> LQFAYKDPE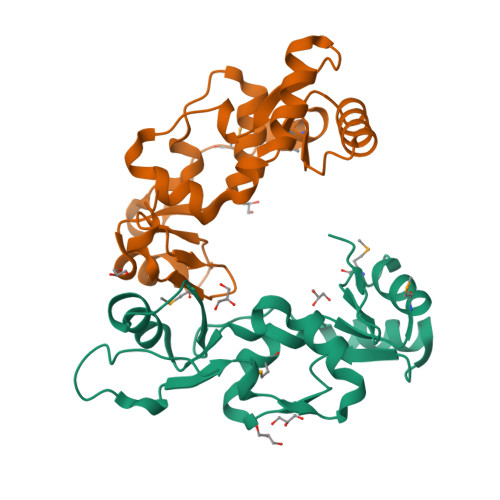KNWNRNSVKGLVASLINVKDNSTATALEVVAGERLYNVVVDTEVTAKKLLEKGELKRRYTIIPLNKISARCIAPETLRVAQNLVGPDNVHVALSLVDYKPELQKGMEFVFGTTFVCNNMDNAKKVAFDKRIMTRTVTLGGDVFDPHGTLSGG;> GKVLDAIIQEKKSGRIPGIYGRLGDLGAIDEKYDIAISSCCHALDYIVVDSIDTAQECVNFLKKHNIGIATFIGLDKMTVWAKKMSKIQTPENTPRLFDLVKVKNEEIRQAFYFALRDTLVANNLDQATRVAYQRDRRWRVVTLQGQIIEQSGTMSGGLEHHHHHH> MKIVYGVIGLILIYIYVSVVSLLFSGIDRKLVARMQRRIGPPILQPFYDFLKLMSKETIIPKTANFMFK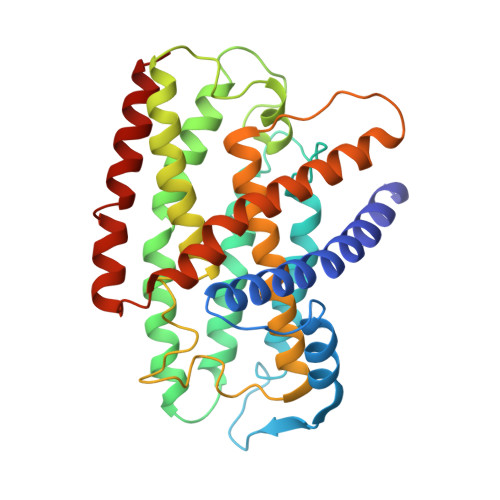AAPILMLATVIALLAYTPLGFPPIFGTKGDIIVFIYLLTLADFFLVVGVMSSGSPYGRIGAARGIALLVSREPAMMLGVFAVMWAISKLGVEKPFSLSSLYEHTIWDFGPVAWVAGVVLIYVFMAWLASEIEVGFFNIPEAEQEIAEGTLVEYSGRYLGIIKLAESIKEFIAASLVVAVLFPWQLNIPGVQGYLINLLLHTLKVFIVLLVSKTIFRTITGRLKISQAVNLLWTRVFTASVIGALLLALGVML> VLFQGPAMSLIPRTERAAFLITPTSYGKSVLGAPLLYFPAQVESNSRGLILAGTHGDETASI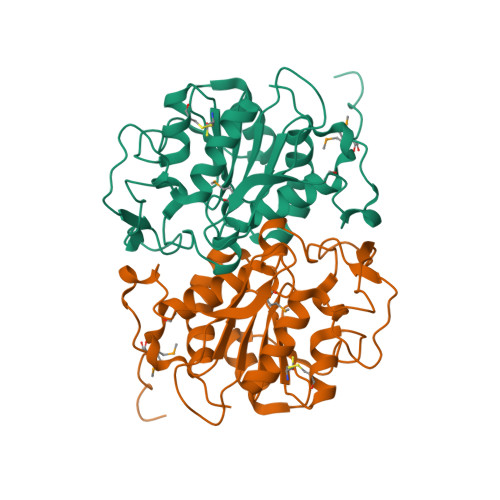AGLSCALRSLPAECLKHDVILSMNPDANQLGTRANANQVDLNRAFPTQNWTEHGTVYRWSSHTPVRDVKVKTGDKEQLEPEVDALISLIELRRPKFVVSFHEPLAFVDDPAHSDLAKWLGKQFNLPIVDDVDYETPGSFGTWCNERQLPCITVELPPISADLTIEKHLDAFIALLQHDPDL>MAKNKVLGRGLADIFPEINEVYEQGLYERANRVVELGIDEVMPNPYQPRKVFSEDSLEELAQSIKEHGLLQPVLVVSENGRYHLIAGERRLRASKLAKMPTIKAIVVDIEQEKMREVALIENIQREDLNPLELARSYKELLESYQMTQEELSKIVKKSRAHVANIMRLLTLSSKVQNALLEEKITSGHAKVLVGLDG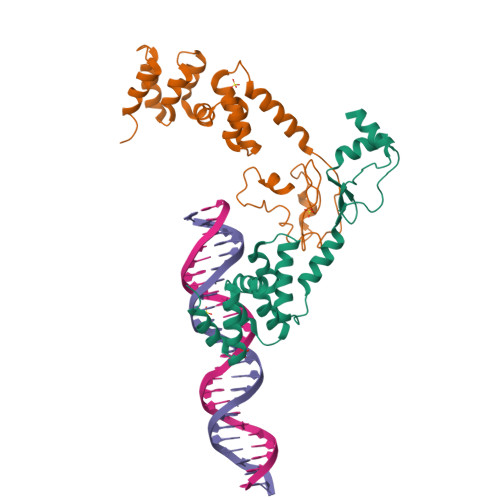EKQELILNSIIGQKLSVRQTEDLARDFKINANFDNKKHGFKQT[4x]>[4x]MSKGRDILTKTIILALREVAPGLEAVLEAHLRATLN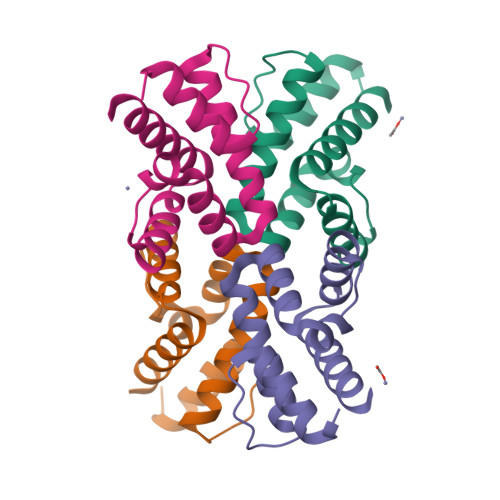SGIELAYDDPQKFKEAVSKLFGEYSARLLEMVIISKLKGRLGEDIEANSLEELVSEIRKIYGE>MATQHPIGKKTACVVGGTGFVASLLVKLLLQKGYAVNTTVRDPDNQKKVSHLLELQELGDLKIFRADLTDELSFEAPIAGCDFVFHVATPVHFASEDPENDMIKPAIQGVVNVMKACTRAKSVKRVILTSSAAAVTINQLDGTGLVVDEKNWTDIEFLTSAKPPTWGYPASKTLAEKAAWKFAEENNIDLITVIPTLMAGSSLTSDVPSSIGLAMSLITGNEFLINGMKGMQMLSGSVSIAHVEDVCRAHIFVAEKESASGRYICCAANTSVPELAKFLSKRYPQYKVPTDFGDFPPK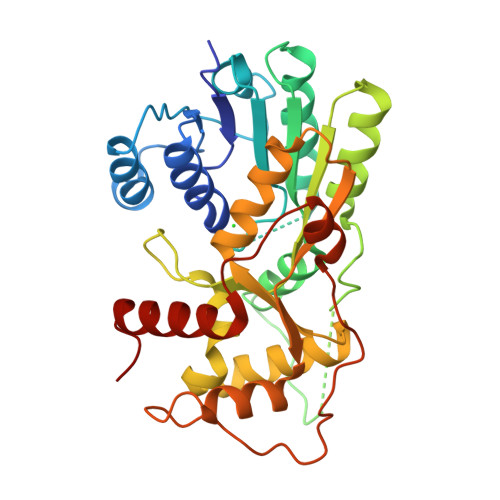SKLIISSEKLVKEGFSFKYGIEEIYDESVEYFKAKGLLQN[2x]In archaea and eukaryotes, the evolutionarily conserved KEOPS is composed of four core subunits―Kae1, Bud32, Cgi121 and Pcc1, and a fifth Gon7/Pcc2 that is found in fungi and metazoa. KEOPS cooperates with Sua5/YRDC to catalyze the biosynthesis of tRNA N6-threonylcarbamoyladenosine (t6A), an essential modification needed for fitness of cellular organisms. We show that A. thaliana KEOPS is composed of KAE1, BUD32, CGI121 and PCC1, which adopts a conserved overall arrangement. PCC1 dimerization leads to a KEOPS dimer that is needed for an active t6A-catalytic KEOPS–tRNA assembly.

Alternatively, a mixture of freshly purified AtKEOPS and AttRNAArgCCU (at a molar ratio of 1:2) was applied to cryo-EM grids for structural analysis. With 232 232 picks, we determined a map of AtKEOPS at an overall resolution of 3.2–5.5 Å. The reconstruction shows six KEOPS subunits―KAE1, PCC1, PCC1, KAE1, BUD32 and CGI121, but no presence of a tRNA molecule. The dissociation of BUD32–CGI121 from KAE1–PCC1 in one KEOPS protomer was probably due to the structural damage at air–water interface during sample preparation. Imposing local refinement, we managed to determine almost a complete structure of AtKEOPS complex with exception for the C-terminal tail of KAE1 (residues 341–353), N-terminal end (residues 1–13) and C-terminal tail (residues 222–226) of BUD32, and N-terminal end of PCC1 (residues 1–15). We modelled a Fe2+ ion in the binding sphere of H113–H117–D298 motif in KAE1 based on crystal structures of Kae1/OSGEP proteins. The final model is composed of a complete AtKEOPS protomer (PCC1–KAE1–BUD32–CGI121) and an incomplete protomer that only contains KAE1–PCC1. In the reconstructed model of AtKEOPS dimer, the two protomers interact via an interacting interface of PCC1 dimer and adopt a V-shaped architecture. In general, the C-lobe of AtBUD32 is located farther away (at least 4 Å) than that of MjBud32 from the C-terminal domain of KAE1. Our structure shows a distance of ∽25 Å between Arg220 of BUD32 and t6A-catalytic site of KAE1.

>[2x]MKKKMIAIGFEGSANKIGVGIVTLDGTILANPRHTYITPPGHGFLPRETAHHHLDHVLPLVKSALETSQVTPEEIDCICYTKGPGMGAPLQVSAIVVRVLSQLWKKPIVAVNHCVAHIEMGRVVTGADDPVVLYVSGGNTQVIAYSEGRYRIFGETIDIAVGNCLDRFARVLKLSNDPSPGYNIEQLAKKGENFIDLPYAVKGMDVSFSGILSYIETTAEEKLKNNECTPADLCYSLQETVFAMLVEITERAMAHCDKKDVLIVGGVGCNERLQEMMRTMCSERDGKLFATDDRYCIDNGAMIAYTGLLAFVNGIETPIEDSTFTQRFRTDEVHAVWREKEAVLLGDKKVAAN;> MDCEENVRDESLVLIKQGAEARVFESTFAGRRSIVKERFSKKYRHPILDAKLTLKRLNAEARCMTKARKLGVCTPVLYAVDTLLHSLTLEYIEGVSVKDIFLEFGTNGVVEERLDDVAAQIGAAIAKLHDGGLAHGDLTTSNMLVRSGTNQLVLIDFGLSVTSTLPEDKAVDLYVLERALLSMHSSCGNVMDRILTAYRKSSKQWSATFNKLAQVRQRGRKRTMIG;> MKVFNLDRGNTLSVSLFSGVTNSKELLNSMLDGSLKLEVSFLNASLIPDIFPLLAAAQKALISKSRDSLSTRTLHSELVYNYSGSKHITESLKRCGISENTTYILAARFNASPVEMEEVAKLINGKEIDLEELKTHANQANILKHYKITSQELGISSLGDAIVCRIAARDALHHHHHH;>[2x]MAATVPATTRSDQTWDFSCNLDVSFESEEHALIAYTSLAVDKELQPDKVRRVMSVSNNKLSVHFEAIEARLLRASFSAFVDVLTLATRTIQEFGQKHHHHHH>MGKHHHHHHGGGDYKDDDDKGSGHMSDKPIDIQYDKQATPNLSGVITPPTNETGNDSVREKLSKLVGDAMSNNPYFAAGGGLMILGTGLAVARSGIIKASRVLYRQMIVDLEIQSKDKSYAWFLTWMAKHPQRVSRHLSVRTNYIQHDNGSVSTKFSLVPGPGNHWIRYKGAFILIKRERSAKMIDIANGSPFETVTLTTLYRDKHLFDDILNEAKDIALKTTEGKTVIYTSFGPEWRKFGQPKAKRMLPSVILDSGIKEGILDDVYDFMKNGKWYSDRGIPYRRGYLLYGPPGSGKTSFIQALAGELDYNICILNLSENNLTDDRLNHLMNNMPERSILLLEDIDAAFNKRSQTGEQGFHSSVTFSGLLNALDGVTSSEETITFMTTNHPEKLDAAIMRPGRIDYKVFVGNATPYQVEKMFMKFYPGETDICKKFVNSVKELDITVSTAQLQGLFVMNKDAPHDALKMVSSLRNANHIF[7x]

For bc1 complex (complex III) assembly, the iron–sulfur protein Rip1 must first be imported into the mitochondrial matrix to fold and acquire its 2Fe–2S cluster, then translocated and inserted into the inner mitochondrial membrane (IM). This translocation of folded Rip1 is accomplished by Bcs1, an unusual heptameric AAA ATPase that couples ATP hydrolysis to translocation. Here, contrary to most AAA-ATPases that form hexameric rings with rather narrow central pores, Bcs1 was shown to form heptameric rings with a significantly wider pore and two large vestibules. One protomer consists of three domains, a transmembrane helix (TMH) at the N-terminus, a Bcs1-specific β-sheet-containing middle domain and a C-terminal AAA cassette.

Here, we were able to distinguish two conformations of Bcs1 after 3D classification that differed from previously observed yBcs1 classes. Notably, our reconstructions showed a substantially narrowed matrix vestibule of ~20 Å in diameter as opposed to ~40 Å and ~30 Å in the ADP or apo states, respectively. This dimension is incompatible with substrate binding at the matrix side and coincided with a wide-open seal ring of 30 Å diameter (only 15 Å in the ADP and Apo1 states) large enough to accommodate Rip1 during translocation. Moreover, the basket TM helices are in a defined position and clearly resolved in ATPγS1, occupying a similar position as observed in yeast ADP or Apo1 states, tightly held together by a hydrophobic seal in IMS leaflet of the IM. The two ATPγS states can be distinguished from each other mainly by the orientation of the middle versus the AAA domains. While the conformation of the AAA domains is essentially the same, we observed a rotation of the middle domains of 6° degrees against the AAA domains, leading to a shift of the middle domains by 7 Å away from the AAA domain in each protomer. Of note, in ATPγS1, the CH forms a contact with the large AAA domain of the neighboring protomer (D124/N125 of the CH with K250 and S253 of AAA), but this contact breaks after the transition to ATPγS2, concomitantly leading to a higher flexibility of the CH loop. ATP binding results in at least two intermediates, here described as ATPγS1 and ATPγS2. We propose that the first intermediate, that we never observe with a bound Rip1, may occur only at an early stage of the translocation.Plasmid-based extended-spectrum AmpC enzymes, such as the FOX β-lactamases, are increasingly found in clinical isolates from antibiotic-resistant infections. FOX-4 is of interest because it rapidly hydrolyzes cephamycins. The first generation of BATSIs inactivated serine β-lactamases (Ambler classes A, C, and D) through a dative and reversible covalent bond to the active site serine nucleophile. In this analysis, the structure of FOX-4 in complex with SM23 and LP06, a ceftazidime mimic, is described.

SM23, a chiral cephalothin (CEF)-based BATSI, bears an R1 side chain with a thiophene ring and an R2 side chain with a m-carboxyphenyl functionality. While apo enzyme crystals contain one FOX-4 chain per asymmetric unit, SM23 (CEF analog) complex crystals contain two chains per asymmetric unit with an RMSD of 0.27 (0.52) Å between Cα (all) atoms. The boron covalently binds to S64. The two boronate oxygens adopt positions consistent with all prior BATSI structures in class C enzymes; one oxygen points into the oxyanion hole and the other takes the presumed position of the deacylating water. The carboxyphenyl ring of SM23 (CEF analog) binds in the canonical binding site of cephalosporins, via hydrogen bonds between the carboxylate, S318, and N343 that are mediated by water molecules. The BATSI carboxyphenyl ring appears to form parallel-displaced π-stacking interactions with the side chain of F293, a residue that is unique to the FOX family. Additionally, the thiophene ring extends out of the active site and does not make significant contacts; instead, it veers away from the Y221 side chain. Overall, the SM23 (CEF analog) adopts a similar shape in both FOX-4 and the E. coli AmpC, with the positioning differences apparently linked to the side chain conformation of L119 and the steric bulk of F293 versus L293. Notably, the amide carbonyls in both structures point toward N152 in spite of these side chain differences, suggesting a common requirement for binding. Since the carboxylate of the carboxyphenyl ring of SM23 (CEF analog) binds in the canonical region consisting of S318, N343, and R349 in FOX-4, this interaction may be the most significant one for increasing binding affinity.

>[2x]GHMSGEAPLTATVDGIIQPMLKAYRIPGMAVAVLKDGKAHYFNYGVANRESGQRVSEQTLFEIGSVSKTLTATLGAYAAVKGGFELDDKVSQHAPWLKGSAFDGVTMAELATYSAGGLPLQFPDEVDSNDKMQTYYRSWSPVYPAGTHRQYSNPSIGLFGHLAANSLGQPFEQLMSQTLLPKLGLHHTYIQVPESAMANYAYGYSKEDKPIRATPGVLAAEAYGIKTGSADLLKFVEANMGYQGDAALKSAIALTHTGFHSVGEMTQGLGWESYDYPVTEQVLLAGNSPAVSFQANPVTRFAVPKAMGEQRLYNKTGSTGGFGAYVAFVPARGIAIVMLANRNYPIEARVKAAHAILSQLAE>[2x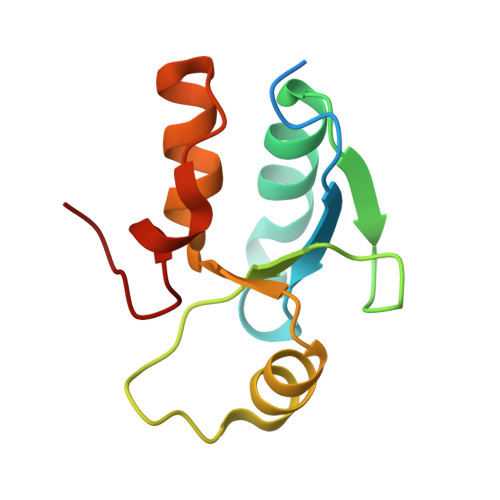]GHMEAQSEKEEAPKPLHKVVVCVSKKLSKKQSELNGIAASLGADYRRSFDETVTHFIYQGRPNDTNREYKSVKERGVHIVSEHWLLDCAQECKHLPESLYPHTYNGS>[2x]MIQFSINRTLFIHALNTTKRAISTKNAIPILSSIKIEVTSTGVTLTGSNGQISIENTIPVSNENAGLLITSPGAILLEASFFINIISSLPDISINVKEIEQHQVVLTSGKSEITLKGKDVDQYPRLQEVSTENPLILKTKLLKSIIAETAFAASLQESRPILTGVHIVLSNHKDFKAVATDSHRMSQ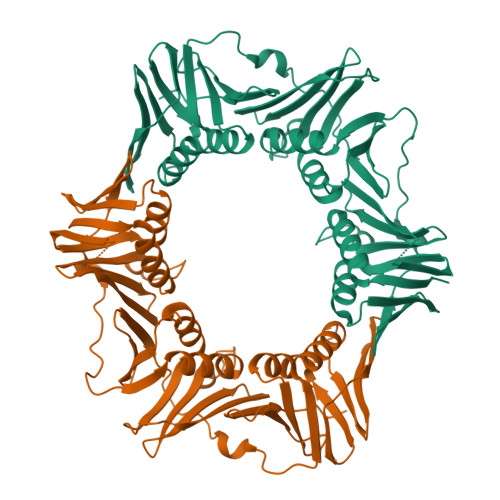RLITLDNTSADFMVVLPSKSLREFSAVFTDDIETVEVFFSPSQILFRSEHISFYTRLLEGNYPDTDRLLMTEFETEVVFNTQSLRHAMERAFLISNATQNGTVKLEITQNHISAHVNSPEVGKVNEDLDIVSQSGSDLTISFNPTYLIESLKAIKSETVKIHFLSPVRPFTLTPGDEEESFIQLITPVRTN>[4x]MSTLANLTEVLFRLDFDPDTAVYHYRGQTLSRLQCRTYILSQASQLARLLKPGDRVVLALNDSPSLACLFLACIAVGAIPAVINPKSREQALADIAADCQASLVVREADAPSLSGPLAPLTLRAAAGRPLLDDFSLDALVGPADLDWSAFHRQD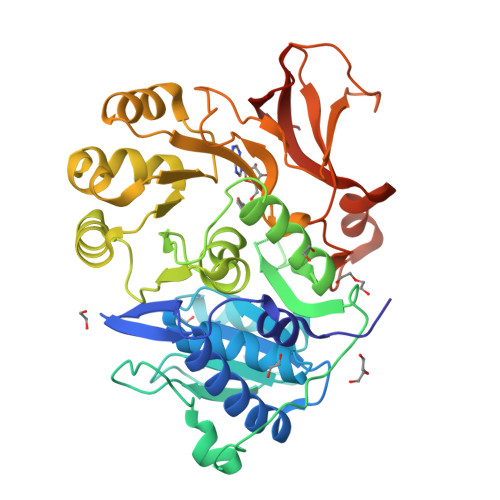PAAACFLQYTSGSTGAPKGVMHSLRNTLGFCRAFATELLALQAGDRLYSIPKMFFGYGMGNSLFFPWFSGASALLDDTWPSPERVLENLVAFRPRVLFGVPAIYASLRPQARELLSSVRLAFSAGSPLPRGEFEFWAAHGLEICDGIGATEVGHVFLANRPGQARADSTGLPLPGYECRLVDREGHTIEEAGRQGVLLVRGPGLSPGYWRASEEQQARFAGGWYRTGDLFERDESGAYRHCGREDLEHHHHHH>SMGRDAPAPAASQPSGCGKHNSPERKVYMDYNATTPLEPEVIQAMTKAMWEAWGNPSSPYSAGRKAKDIINAARESLAKMIGGKPQDIIFTSGGTESNNLVIHSVVKHFHANQTSKGHTGGHHSPVKGAKPHFITSSVEHDSIRLPLEHLVEEQVAAVTFVPVSKVSGQTEVDDILAAVRPTTRLVTIMLANNETGIVMPVPEISQRIKALNQERVAAGLPPILVHTDAAQALGKQRVDVEDLGVDFLTIVGHKFYGPRIGALYIRGLGEFTPLYPMLFGGGQERNFRPGTENTPMIAGLGKAAELVTQNCEAYEAHMRDVRDYLEERLEAEFG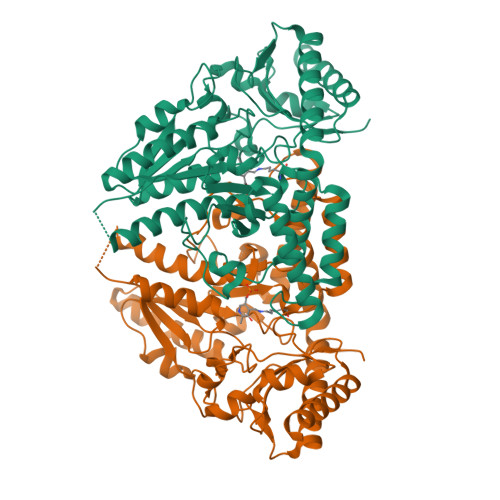QKRIHLNSQFPGTQRLPNTCNFSIRGPRLQGHVVLAQCRVLMASVGAACHSDHGDQPSPVLLSYGVPFDVARNALRLSVGRSTTRAEVDLVVQDLKQAVAQLEDQA[2x]> MSKILVCIKQVPGTSNVEVDPETGVLIRDGVESKLNPYDLFGLETAFRLKEQLGGTITTLSMGPMQSKEVLMESFYMGADEGCLLSDRKFGGADVVATSYTL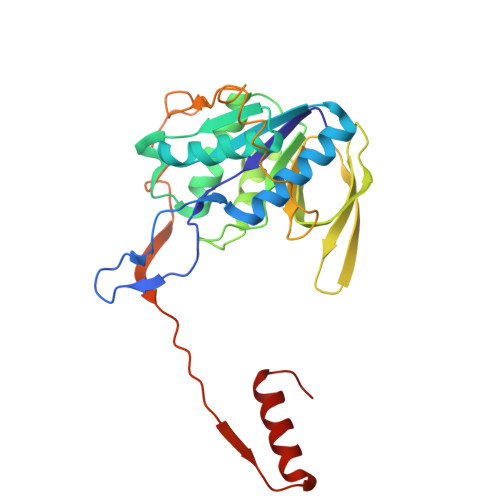AQGTKRLGDFDLIICGKQTTDGDTAQVGPEMAEFLGIPHVTNVIKILAADEKGLTLQMNMEESLEIQRVPYPCLITVDKDIYTPRLPSYKRKLDISKNPEIKILTLKDMYDTNEKKYGLSGSPTQVERIFPPESNVEKTSFEGDGKVLAKALLGILTEKKYLG4-azanyl-6-[[(1~{S})-1-[6-fluoranyl-1-(3-methylsulfonylphenyl)benzimidazol-2-yl]ethyl]amino]pyrimidine-5-carbonitrile 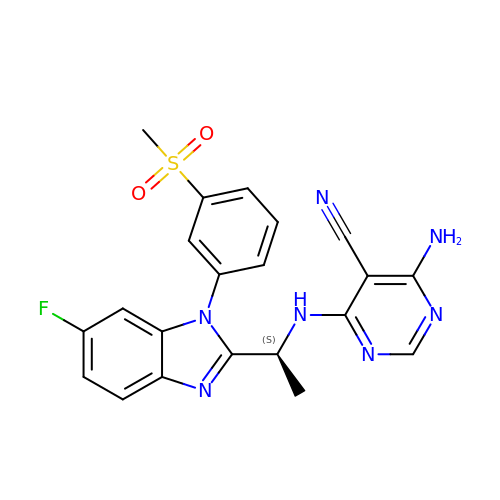| C21 H18 F N7 O2 S | ARGMEIUNNDIMNN-LBPRGKRZSA-N> SHKNRIFVSSSKDFEGYPSKAIVPVQFVALLTSIHLTETKCLLGFSNFERRGDQSQEDQYLIKLKFKDRGSERLARITISLLCQYFDIELPDLDSDSGASPTVILRDIHLERLCFSSCKALYVSKHGNYTLFLEDIKPLDLVSVISTISTKSTNSSKHSSSELISECDLNNSLVDIFNNLIEMNRDEKNRFKFVKLIHYDIELKKFVQDQQKVLSQKSKAAAINPFF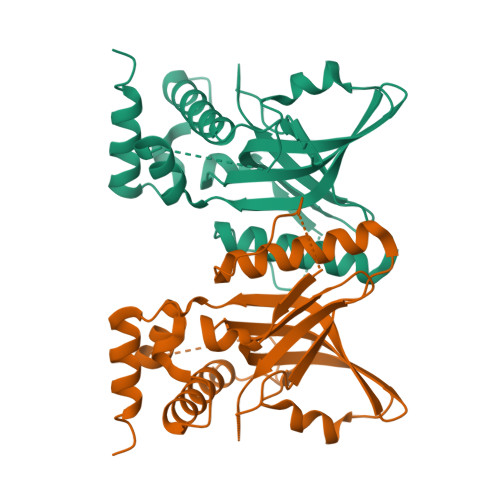VPNRLG>[2x]MSLSLLVIGSLAFDDIETPFGRSDNTLGGSSTYIALSASYFTDEPIRMVGVVGSDFGKEHFDLLHAKNIDTRGIQVIEDGKTFRWAGRYHYDMNTRDTLDTQLNVFAEFDPHVPQYYRDSK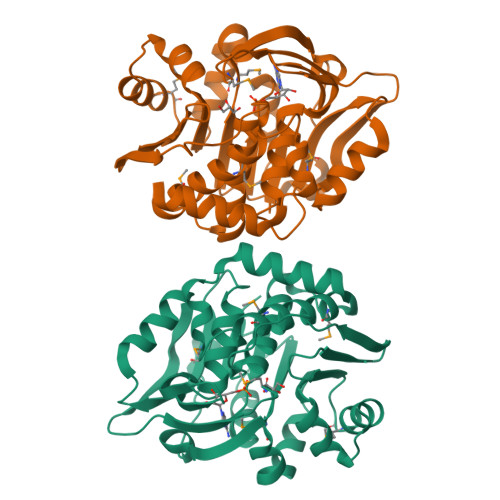FVCLGNIDPELQLKVLDQIDDPKLVVCDTMNFWIEGKPEELKKVLARVDVFIVNDSEARLLSGDPNLVKTARIIREMGPKTLIIKKGEHGALLFTDNGIFAAPAFPLESIYDPTGAGDTFAGGFIGHLARCGNTSEAEMRKAVLYGSAMASFCVEQFGPYRYNDLDLLEVDDRYQSFLELSRIEEGHHHHHH> MNHSAECTCEESLCETLRAFSAQHPESVLYQTSLMSALLSGVYEGSTTIADLLKHGDFGLGTFNELDGELIAFSSQVYQLRADGSARNAQPEQKTPFAVMTWFQPQYRKTFDHPVSRQQLHEVIDQQIPSDNLFCALRIDGHFRHAHTRTVPRQTPPYRAMTDVLDDQPVFRFNQREGVLVGFRTPQH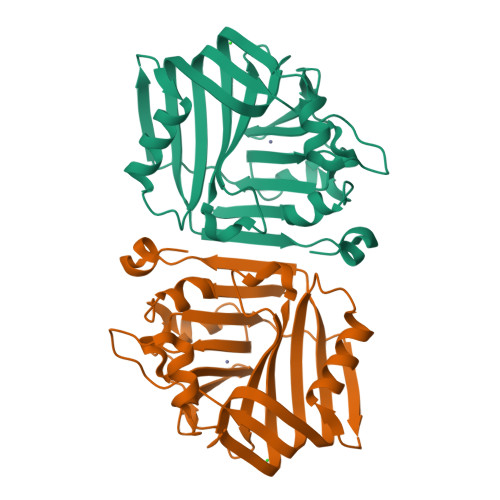MQGINVAGYHEHFITDDRKGGGHLLDYQLDHGVLTFGEIHKLMIDLPADSAFLQANLHPDNLDAAIRSVES> AKQKKEKVWAHYEEQPVEEVMPVLEEKERSASYKPVFVTEITDDLHFYVQDVETGTQLEKLMENMRNDIASHPPVEGSYAPRRGEFCIAKFVDGEWYRARVEKVESPAKIHVFYIDYGNREVLPSTRLGTLSPAFSTRVLPAQATEYAFAFIQVPQDDDARTDAVDSVVRDIQNTQCLLNVEHLSAGCPHVTLQFAD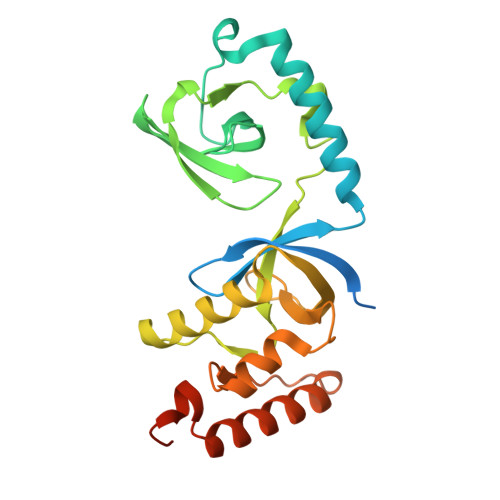SKGDVGLGLVKEGLVMVEVRKEKQFQKVITEYLNAQESAKSARLNLWRYGDFRADDADEFGYSR> GPGSEFCADQYWNEVAVIDAIPLAATEHDTMLEMSDMQVWSAGDHPPIVSEEDISGSLVPRGSGSKSDSNASFLRAARAGNLDKVVEYLKGGIDINTCNQNGLNALHLAAKEGHVGLVQELLGRGSSVDSATKKGNTALHIASLAGQAEVVKVLVKEGANINAQSQNGFTPLYMAAQENHIDVVKYLLENGANQSTATEDGFTPLAVALQQGHNQAVAILLENDTKGKVRLPALHIAARKDDTKSAALLLQNDHNADVQSKMMVNRTTESGFTPLHIAAHYGNVNVATLLLNRGAAVDFTARNGITPLHVASKRGNTNMVKLLLDRGGQIDAKTRDGLTPLHCAARSGHDQVVELLLERGAPLLARTKNGLSPLHMAAQGDHVECVKHLLQHKAPVDDVTLDYLTALHVAAHCGHYRVTKLLLDKRANPNARALNGFTPLHIACKKNRIKVMELLVKYGASIQAITESGLTPIHVAAFMGHLNIVLLLLQNGASPDVTNIRGETALHMAARAGQVEVVRCLLRNGALVDARAREEQTPLHIASRLGKTEIVQLLLQHMAHPDAATTNGYTPLHISAREGQVDVASVLLEAGAAHSLATKKGFTPLHVAAKYGSLDVAKLLLQRRAAADSAGKNGLTPLHVAAHYDNQKVALLLLEKGASPHATAKNGYTPLHIAAKKNQMQIASTLLNYGAETNIVTKQGVTPLHLASQEGHTDMVTLLLDKGANIHMSTK

Ankyrins are a widely expressed scaffold protein family, which mainly function to link great varieties of functionally related but structurally diverse integral membrane proteins to the spectrin-based cytoskeletons. Each ankyrin contains an N-terminal membrane binding domain (MBD), which is composed of 24 ANK repeats and responsible for binding to diverse membrane targets. Following the MBD is an unstructured linker region of ~130 amino acid residues, followed sequentially by a ZU5-ZU5-UPA supramodule responsible for spectrin binding (SBD), a death domain (DD), and an intrinsically disordered C-terminal tail (CT) with varying lengths. We identified three distinct autoinhibitory segments from the intrinsically disordered linker and CT regions of AnkB, and elucidated the inhibition mechanism of these segments by detailed biochemical and structural investigations.

Although AnkB and G do not contain AnkR_CT like sequences in their tails, more thorough sequence analysis revealed that both AnkB and G contain a 13-residue segment (denoted as ‘AI-a’ for the AutoInhibition segment-a) that share a similar sequence pattern with the last 13-residue fragment of AnkR_CT and several MBD ‘site-1’ binding targets such as Na+ and K+-channels. As an alternative approach, we replaced the corresponding sequence of AnkR_CT with that of AnkB_AI-a and produced an AnkR/B_CT Chimera. Isothermal titration calorimetry (ITC) experiments detected a strong interaction between this chimera peptide and AnkB_MBD, with a Kd value comparable to that of AnkR_CT with AnkB_MBD. This chimera peptide was fused to the N-terminus of AnkB_MBD for crystallization trials as we have demonstrated for AnkR_CT. With this strategy, we successfully obtained crystals of the AnkR/B_CT Chimera/AnkB_repeats_R1-20 fusion protein, and the crystals were diffracted up to 3.3 Å. The structure of the fusion protein was determined by the molecular replacement method using the AnkB_repeats_R1-24 structure as the model. Consistent with the biochemical analysis, the structure showed that the AnkB_AI-a segment binds to ‘site-1’ of AnkB_MBD (repeats_R1-5) using essentially the same binding mode as we observed in the AnkR_CT/AnkB_MBD and Nav1.2_ABD/AnkB_R1-9 complex structures. In particular, Glu1630 from AnkB_AI-a occupies the identical position as Glu1622 in AnkR or Glu1112 in Nav1.2 on AnkB_R1-5, by forming strong hydrogen bonds with Thr94 and Asn98 in the R2-R3 finger loop. Additionally, hydrophobic interactions between ‘PPIV’ from AI-a and hydrophobic residues (including the two critical Phe residues, Phe131 and Phe164, from R4 and R5; see Wang et al., 2014) from R3-R5 also contribute to the binding.> AKQRESTDAIFVHCSATKPSQNVGVREIRQWHKEQG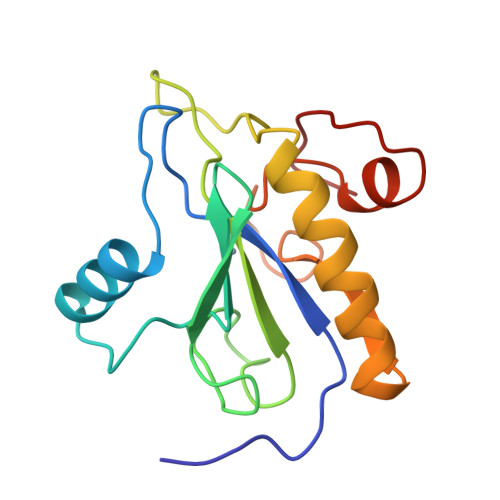WLDVGYHFIIKRDGTVEAGRDEMAVGSHAKGYNHNSIGVCLVGGIDDKGKFDANFTPAQMQSLRSLLVTLLAKYEGAVLRAHHEVAPKACPSFDLKRWWEKNELVTSDRG>MKLSKQKASLLTAVLLLLSLSITTITVDAARVRTYPNVSHANTHYKNTVSSKLLPFTANYQL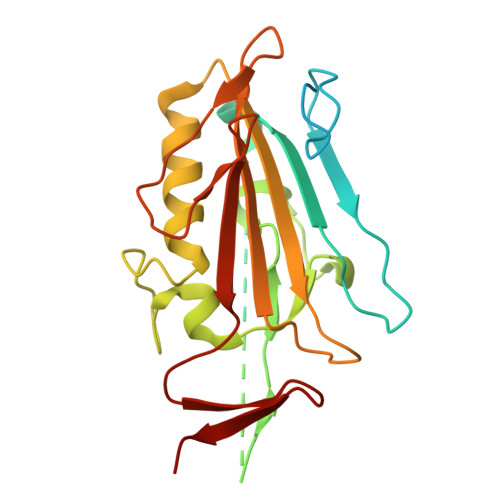QLGELDNLNRATFSHIQLQDRHETKDVRTKINYDPVGWHNYQFPYGDGSKSSWVMNRGHLVGYQFCGLNDEPRNLVAMTAWLATGAYSGANDSNPEGMLYYENRLDSWLALHPDFWLDYKVTPIYSGNEVVPRQIELQYVGIDSSGELLTIRLNSNKESIDENGVTTVILENSAPNINLDYLNGTATPKN[2x]> FPTIP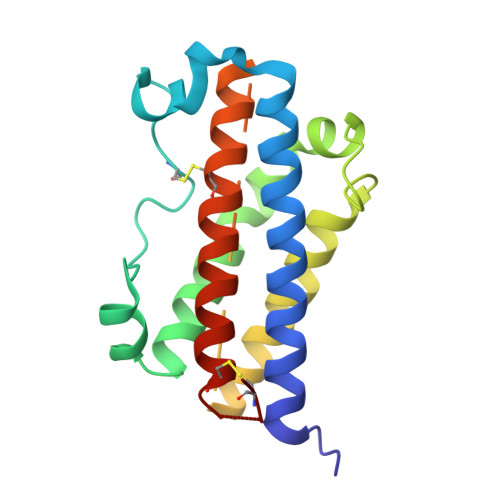LSRLADNAWLRADRLNQLAFDTYQEFEEAYIPKEQIHSFWWNPQTSLCPSESIPTPSNKEETQQKSNLELLRISLLLIQSWLEPVQFLRSVFANSLVYGASDSNVYDLLKDLEEGIQTLMGRLEDGSPRTGQIFKQTYSKFDTNSHNDDALLKNYGLLYCFNKDMSKVSTYLRTVQCRSVEGSCGF>MEMRVLLIAGGVSPEHEVSLLSAEGVLRHIPFPTDLAVIAQDGRWLLGEKALTALEAKAAPEGEHPFPPPLSWERYDVVFPLLHGRFGEDGTVQGFLELLGKPYVGAGVAASALCMDKDLSKRVLAQAGVPVVPWVAVRKGEPPVV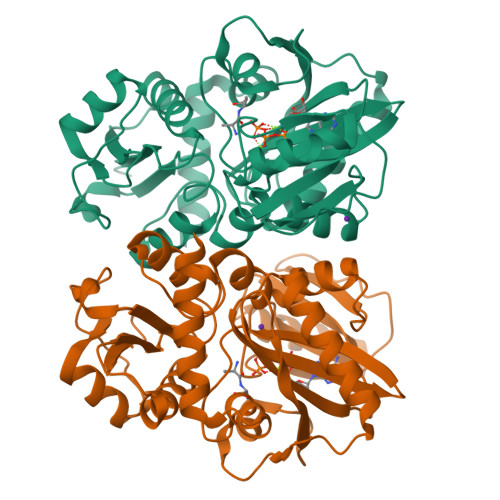PFDPPFFVKPANTGSSVGISRVERFQDLEAALALAFRYDEKAVVEKALSPVRELEVGVLGNVFGEASPVGEVRYEAPFYDYETKYTPGRAELLIPAPLDPGTQETVQELALKAYKVLGVRGMARVDFFLAEGELYLNELNTIPGFTPTSMYPRLFEAGGVAYPELLRRLVELALTHHHHHH[2x]>[2x]MLPKELLDATRRRGKIYLKFASEEHFRLARAVILAFKSSVGQKYEDLQEKLRHMERAENYRKVRGFAKILERESEFTTSSSLDPLEVRRFLFSRGYVTSEIERAKIIAEAATYFNTTPEEIERAMFADREEEKILTRVPGISEEELIRRYNLSLLQTLMFNSARMSFRVSENHKRIFRLIKLLGLMYEIS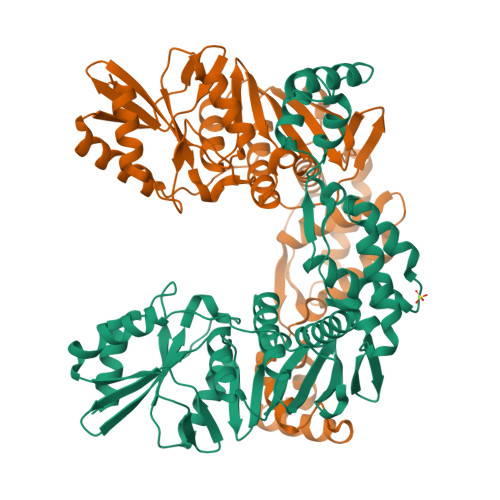GENIEITGPASILKMTRKYGTSMAKLIPEIVKAKEWAIKAEIIEDKRVYFFELSSEDDILLPKLEVSVEYDSSLEREFVTKIKRILGVEVIREPGIIKAGQYAYIPDFLIRKNGKEVYVEIAGFWTRSYIKSKLEKLSNVDVKMLIIVNDELLADKLGKIHDVIVMRKGKIPYKEVILKLKEMLN> MTDNHIDVLINGCGIGGAMLAYLLGRQGHRVVVVEQARREYARNRADLLKPAGIRVVEAAGLLAEVTRRGGRVRHELEVYHDGELLRYFNYSSVDARGYFILMPGESLRRLVLEKIDGEATVEMLFETRIEAVQRDERHAIDQVRLNDGRVLRPRVVVGADGIASYVRRRLLDIDVERRPYPSPMLVGTFALAPCVAERNRLYVDSQGGLAYFYPIGFDRARLVVSFPREEARELMADTRGESLRRRLQRFVGDESAEAIAAVTGTSRFKGIPIGYLNLDRYWADNVAMLGDAIHNVHPITGQGMNLAIEDASALADALDLALRDACALEDALAGYQAERFPVNQAIVSYGHALATSLEDRQRFAGVFDTALQGSSRTPEALGGERSYQPVRSPAPLG

In this study, we show that the catalytic activity of the flavoprotein monooxygenase (FPMO) PqsL can be triggered by blue-light illumination. The enzyme is involved in the biosynthesis of 2-alkyl-4-hydroxyquinoline N-oxides (AQNO) in the opportunistic pathogen Pseudomonas aeruginosa. It is homologous to group A FPMOs13 and has a relatively high similarity to p-hydroxybenzoate hydroxylase (pHBH), the most thoroughly studied FPMO14. In contrast, PqsL catalyzes the hydroxylation of an aromatic-amine group, a rather uncommon reaction, and remarkably shows no intrinsic catalytic activity with NAD(P)H as cosubstrate.

To render PqsL accessible to more demanding applications and analyses, we used a rational design approach, generating an enzyme variant with stronger FAD binding and thus improved stability. Our starting point was the observation that PqsL displays a deviation in its FAD-binding site where Gly45 replaces an arginine side chain mostly conserved in pHBH-related enzymes. Specifically, the equivalent Arg44 of pHBH anchors the pyrophosphate group of the FAD. The crystal structure of the PqsL-Q mutant revealed some local changes in the conformation of the 40-46 loop and confirmed that, as intended, Arg45 (replacing Gly45 of the wild-type) does engage the FAD pyrophosphate, which explains the 7-fold lower KD of FAD displayed by the mutant as compared to the wild-type protein (37.5 ± 6.7 nM vs 249.5 ± 29.8 nM, respectively). The increased affinity for FAD likely explains another favorable feature of the mutant protein: purified PqsL-Q exhibited an increased thermostability and no degradation at room temperature. Moreover, the flavin of the mutant protein is slightly shifted outward with respect to the wild-type conformation. We also found that neither cosubstrate specificity, substrate affinity nor KM values profoundly differ between PqsL and PqsL-Q, even though amino acid exchanges in PqsL-Q included positions designated to NADPH binding. The photoactivated reductive half reaction was assayed by NAD(P)H oxidation kinetics and revealed approximately 67% of wild-type activity. On the other hand, we can conclude that the more rigid conformation in which FAD is coordinated by PqsL-Q apparently does not hinder the photocatalytic reaction. Using an engineered variant of PqsL, we further demonstrate that stabilization of the protein-cofactor complex does not diminish photoreactivity, indicating that primarily the conformation of the flavin ring and its microenvironment are relevant for photoreduction.>TPAFNKPKVELHVHLDGAIKPETILYFGKKRGIALPADTVEELRNIIGMDKPLSLPGFLAKFDYYMPVIAGCREAIKRIAYEFVEMKAKEGVVYVEVRYSPHLLANSKVDPMPWNQTEGDVTPDDVVDLVNQGLQEGEQAFGIKVRSILCCMRHQPSWSLEVLELCKKYNQKTVVAMDLAGDETIEGSSLFPGHVEAYEGAVKNGIHRTVHAGEVGSPEVVREAVDILKTERVGHGYHTIEDEALYNRLLKENMHFEVCPWSSYLTGAW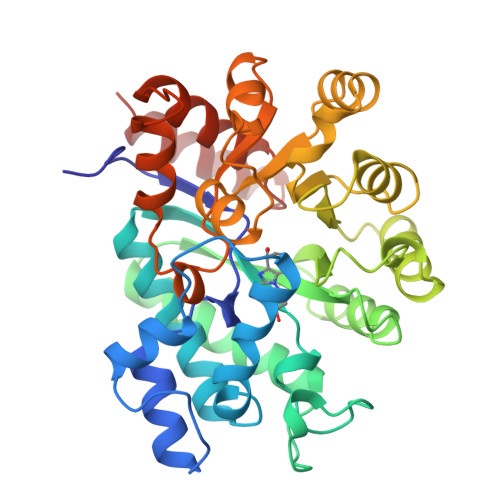DPKTTHAVVRFKNDKANYSLNTDDPLIFKSTLDTDYQMTKKDMGFTEEEFKRLNINAAKSSFLPEEEKKELLERLYREYQ[4x]> MTTPPVVANYENASMAADYIKRVSNVLPDIGIICGSGLGKLIEEIEERKVIPYINIPNFPKTTVAGHVGNLVLGSVGGRKIVAMQGRLHMYEGYSNQEIALPIRVMKLLGVRVLLITNLAGGINRKLKSGDFVLIKGHINFPGLGLNNVLVGPNQDEFGPRFPDLSNAYDRLLQQLALKIAQENDFQDLVHEGVYAFNGGPTYESPDESNMLLKLGCDVVGMSTVPEVIIACHCGIKVLAVSLIANNSILDAENDVSI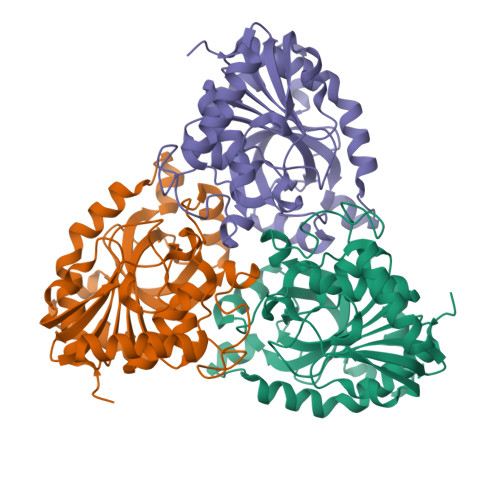NHEKVLAVAEKRADLLQMWFKEIITRLPLD>GPLGSMSTLDLNHLADLYDRKDWNACKKELLKLKVELAKQNLFVPTSDKEKASFARNVFEYGVLVSIQTCDIESFARYASQVIPFYHDSLVPSSRMGLVTGLNLLYLLSENRIAEFHTALESVPDKSLFERDPYVEWVISLEQNVMEGAF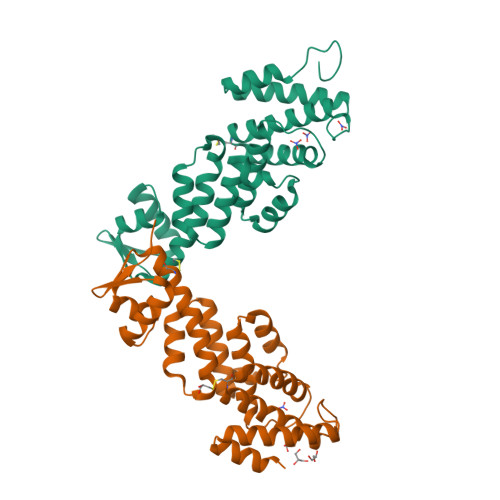DKVASMIRSCNFPEFSYFMKIVMSMVRNEIATCAEKVYSEIPLSNATSLLYLENTKETEKLAEERGWDIRDGVIYFPKE[2x]Hyp-1, the protein product (comprised of 159 residues) of the hyp-1 gene in Hypericum perforatum has a picturesque history. That study, however, could never be replicated and instead the crystal structure of the Hyp-1 protein revealed the canonical PR-10-fold strongly suggesting classification in class 10 of the superfamily of plant Pathogenesis-Related (PR-10) proteins. The characteristic PR-10-fold, also known as the Betv1 fold according to the first protein from this class, a birch (Betula verucosa) pollen allergen to have its crystal structure determined, consists of a large seven-stranded antiparallel β-sheet forming a baseball-glove grip over a long C-terminal helix α3, which is the most variable element of the PR-10 structure. In the case of Hyp-1, we observe two separated internal chambers (1 and 2), each with its own entrance (E1 and E2, respectively), and a third site (3) which is formed as a deep invagination of the protein surface.

In this work we present high resolution crystal structure of Hyp-1 in complex with melatonin, demonstrating that this physiological ligand utilizes the same internal docking sites as ANS. The Hyp-1/MEL structure is the first example reported in the Protein Data Bank (PDB) of melatonin bound to a plant protein, and the second case with any protein, the first one being human quinone reductase. Careful examination of difference electron density maps revealed the positions of 204 water molecules as well as of two molecules of MEL, one of which (modeled in two orientations, with average B-factor of 54.5 Å2) is most likely endowed with rotational degrees of freedom within the surface invagination, and another one (modeled in one orientation with of 36.1 Å2) is well stabilized in the internal cavity of the protein. In addition, there are three Na+ ions included in the model, two of which are octahedrally coordinated by the protein (one by loop L5 and another one by strand β1 and the C-end of helix α3), and a third one partially occupied within the protein cavity. The MEL molecule at site 1 that has the best definition in electron density, makes direct contacts with the protein only via weak (3.6–3.8 Å) hydrophobic interactions with Phe39, Leu31, Leu65, Val91, Gly136, and Lys139, as well as via water-mediated hydrogen bonds of its O21 atom with Gly136 (O), Ala140 (N), and Met68 (Sδ), and of its N1 atom with Arg93 (Nη2) and Glu132 (O). Interestingly, the MEL1 ligand is additionally stabilized and pushed to its binding site by a direct hydrogen bond of its N2 atom with the carboxylate group of Asp48 from loop L4 of an adjacent Hyp-1 molecule. The MEL3 ligand is evidently rotating between the jaws of the vise formed by the side chains of Lys33 and Tyr150. Although we did not model melatonin at site 2, it is quite obvious that the electron density there is consistent with the shape of the indole ring. The three binding sites identified in the Hyp-1/MEL complex are exactly the same as in the Hyp-1/ANS complex.

> GIDPFTMAAYTIVKEEESPIAPHRLFKALVLERHQVLVKAQPHVFKSGEIIEGDGGVGTVTKITFVDGHPLTYMLHKFDEIDAANFYCKYTLFEGDVLRDNIEKVVYEVKLEAVGGGSKGKITVTYHPKPGCTVNEEEVKIGEKKAYEFYKQVEEYLAANPEVFA In this paper, we describe the molecular architecture of the prototypical bacterial SNARE-like protein IncA, which mediates the homotypic fusion of chlamydial inclusions. IncA is a protein of 273 amino acids composed of a short, cytoplasmic N-terminal moiety (residues 1–34), a bilobed transmembrane domain (residues 35–84), and a long cytoplasmic C-terminal domain that ends in a tail with low complexity (residues 247–273). We demonstrate that IncA folds into a stable, non-canonical four-helix bundle that is maintained as a monomer by intramolecular interactions. Cells infected with an IncA-deficient strain of C. trachomatis similarly displayed multiple inclusions at a high multiplicity of infection, further establishing that IncA is required for the homotypic fusion of inclusions.

To better understand the mechanism of IncA-mediated membrane fusion, we generated high-quality crystals of a chymotryptic fragment of IncA spanning residues 87–246 (IncA87–246) and determined a crystal structure of IncA87–246 to an Rwork/free of 14.1/16.8% at 1.12 Å resolution. The electron density for IncA87–246, including the six N-terminal histidines of the affinity tag, is exceptionally clear, consistent with the low B-factor of the crystal structure (~10.8 Å2). We found that IncA87–246 adopts an asymmetric and slightly blocky conformation, somewhat similar to a four-helix bundle. Both in crystal and in solution, IncA87–246 exists as a monomer, as previously observed for the full-length cytosolic domain of IncA (ΔTMD-IncA - Supplementary Fig. 1a), that sediments at equilibrium as a single species of 23.9 ± 0.8 kDa8. The tertiary structure of IncA87–246 consists of four down-up-down-up antiparallel α-helices, named HA-HD. However, IncA87–246 deviates from canonical four-helix bundles in at least three aspects. First, the helix HB is interrupted at position 144 by a glycine that generates two shorter helices, named HB’ and HB”. Third, while helices HA and HC run parallel to each other making an acute angle of ~ 10° and bonding throughout their entire length, the longest helix HD makes a 40° angle from helix HC pointing away from the Hclamp and gives an asymmetric appearance to the helical bundle. The hinge and the amino acids preceding Hclamp were found to have significantly higher than average B-factors (~ 26 Å2 vs. ~ 16 Å2), possibly underscoring intrinsic flexibility. Our simulations showed that the structure of IncA87–246 is highly stable and is unlikely to be a metastable intermediate.

> ATANLHLYQDLQREVGSLKEINFMLSVLQKEFLHLSKEFATTSKDLSAVSQDFYSCLQGFRDNYKGFESLLDEYKNSTEEMRKLFSQEIIADLKGSVASLREEIRFLTPLAEEVRRLAHNQQSLTAAIEELKTIRDSLRDEIGQLSQLSKTLTSQIALQRKLEHHHHHH(2~{S},4~{S})-2-ethoxycarbonyl-5,5-dimethyl-2-(sulfanylmethyl)-1,3-thiazolidine-4-carboxylic 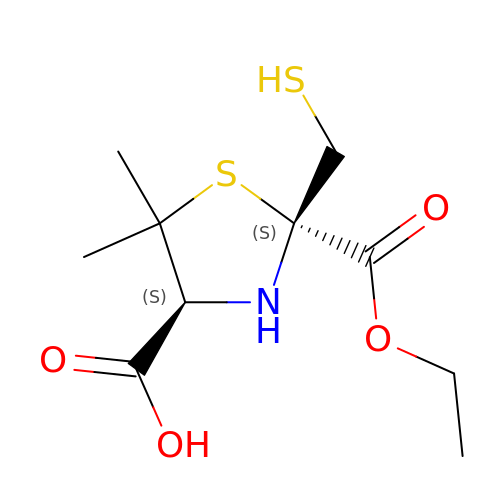acid | C10 H17 N O4 S2 | PUOMKKVEJFJZFE-QUBYGPBYSA-N> KRNKPGKATGKGKPVNNKWLNNAGKDLGSPVPDRIANKLRDKEFKSFDDFRKKFWEEVSKDPELSKQFSRNNNDRMKVGKAPKTRTQDVSGKRTSFELHHEKPISQN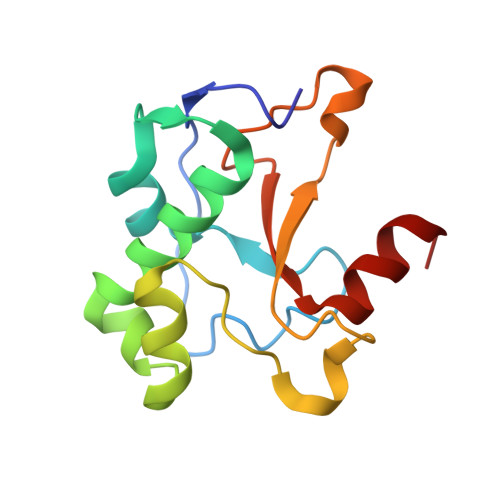GGVYDMDNISVVTPKRHIDIHRGK>[8x]M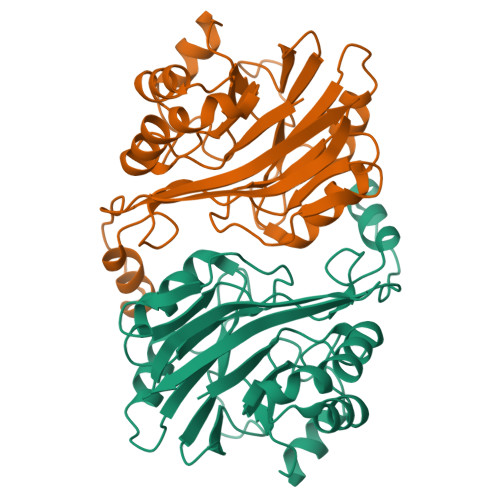RVLFIGDVFGQPGRRVLQNHLPTIRPQFDFVIVNMENSAGGFGMHRDAARGALEAGAGCLTLGNHAWHHKDIYPMLSEDTYPIVRPLNYADPGTPGVGWRTFDVNGEKLTVVNLLGRVFMEAVDNPFRTMDALLERDDLGTVFVDFHAEATSEKEAMGWHLAGRVAAVIGTHTHVPTADTRILKGGTAYQTDAGFTGPHDSIIGSAIEGPLQRFLTERPHRYGVAEGRAELNGVALHFEGGKATAAERYRFIED1-[4-(3-methyl-4-phenyl-phenyl)carbonyl-1,4-diazepan-1-yl]ethanone 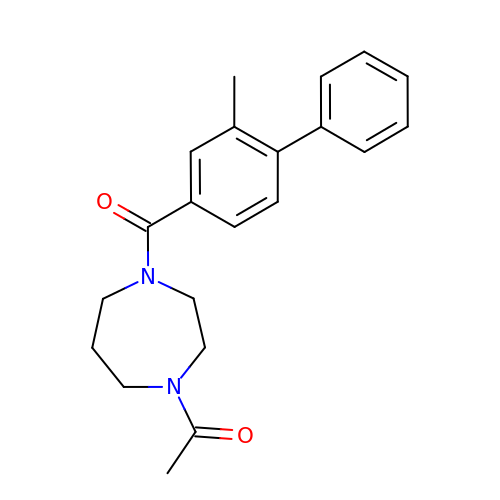| C21 H24 N2 O2 | FIBAYMYQCFMKFA-UHFFFAOYSA-N> TAVVQRVEIHKLRQGENLILGFSIGGGIDQDPSQNPFSEDKTDKGIYVTRVSE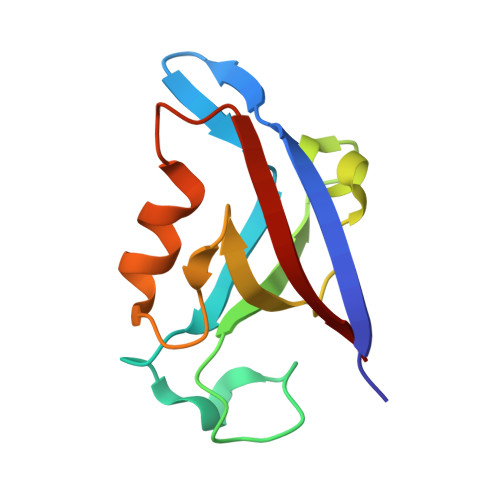GGPAEIAGLQIGDKIMQVNGWDMTMVTHDQARKRLTKRSEEVVRLLVTRQ>[2x]MVGLIWAQATSGVIGRGGDIPWRLPEDQAHFREITMGHTIVMGRRTWDSLPAKVRPLPGRRNVVLSRQADFMASGAEVVGSLEEALTSPETWVIGGGQ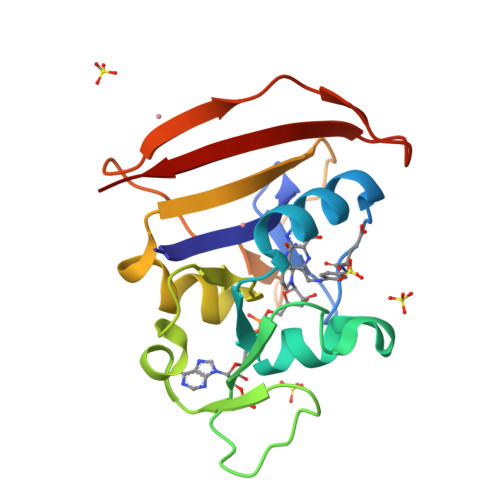VYALALPYATRCEVTEVDIGLPREAGDALAPVLDETWRGETGEWRFSRSGLRYRLYSYHRS> SSLDDKPQFPGASAEFIDKLEFIQPNVISGIPIYRVMDRQGQIINPSEDPHLPKEKVLKLYKSMTLLNTMDRILYESQRQGRISFYMTNYGEEGTHVGSAAALDNTDLVFGQYREAGVLMYRDYPLELFMAQCYGNISDLGKGRQMPVHYGCKERHFVTISSPLATQIPQAVGAAYAAKRANANRVVICYFGEGAASEGDAHAGFNFAATLECPIIFFCRNNGYAISTPTSEQYRGDGIAARGPGYGIMSIRVDGNDVFAVYNATKEARRRAVAENQPFLIEAMTYRIGHHNTSDDSSAYRSVDEVNYWDKQDHPISRLRHYLLSQGWWDEEQEKAWRKQSRRKVMEAFEQAERKPKPNPNLLFSDVYQEMPA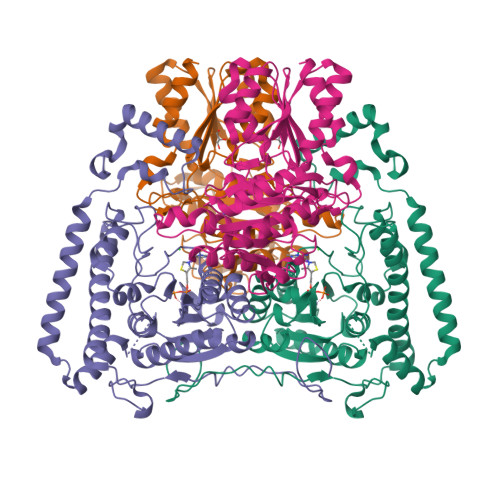QLRKQQESLARHLQTYGEHYPLDHFDK;> VAHFTFQPDPEPREYGQTQKMNLFQSVTSALDNSLAKDPTAVIFGEDVAFGGVFRCTVGLRDKYGKDRVFNTPLCEQGIVGFGIGIAVTGATAIAEIQFADYIFPAFDQIVNEAAKYRYRSGDLFNCGSLTIRSPWGCVGHGALYHSQSPEAFFAHCPGIKVVIPRSPFQAKGLLLSCIEDKNPCIFFEPKILYRAAAEEVPIEPYNIPLSQAEVIQEGSDVTLVAWGTQVHVIREVASMAKEKLGVSCEVIDLRTIIPWDVDTICKSVIKTGRLLISHEAPLTGGFASEISSTVQEECFLNLEAPISRVCGYDTPFPHIFEPFYIPDKWKCYDALRKMINY>GSHMKVLLLGFEFLPVKVGGLAEALTAISEALASLGHEVLVFTPSHGRFQGEEIGKIRVFGEEVQVKVSYEERGNLRIYRIGGGLLDSEDVYGPGWDGLIRKAVTFGRASVLLLNDLLREEPLPDVVHFHDWHTVFAGALIKKYFKIPAVFTIHRLNKSKLPAFYFHEAGLSELAPYPDIDPEHTGGYIADIVTTVSRGYLIDEWGFFRNFEGKITYVFNGIDCSFWNESYLTGSRDERKKSLLSKFGMDEGVTFMFIGRFDRGQKGVDVLLKAIEILSSKKEFQEMRFIIIGKGDPELEGWARSLEEKHGNVKVITEMLSREFVRELYGSVDFVIIPSYFEPFGLVALEAMCLGAIPIAS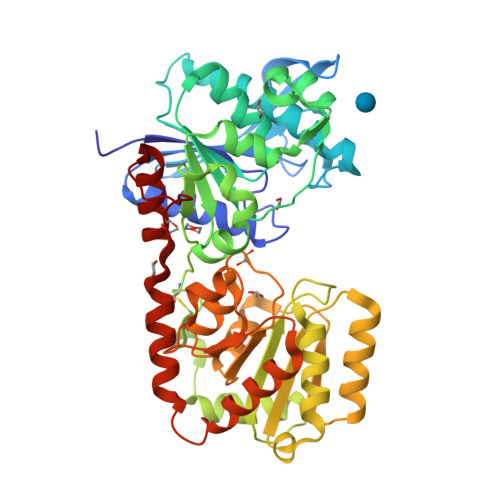AVGGLRDIITNETGILVKAGDPGELANAILKALELSRSDLSKFRENCKKRAMSFSWEKSAERYVKAYTGSIDRAFDFIL[3x]> CGRTSCHLPRDVLTRACAYQDRRGQQRLPEWRDPDKYCPSYNKSPQSNSPVLLSRLHFEKDADSSERIIAPMRWGLVPSWFKESDPSKLQFNTTNCRSDTVMEKRSFKVPLGKGRRCVVLADGFYEWQRCQGTNQRQPYFIYFPQIKTEKSGSIGAADSPENWEKVWDNWRL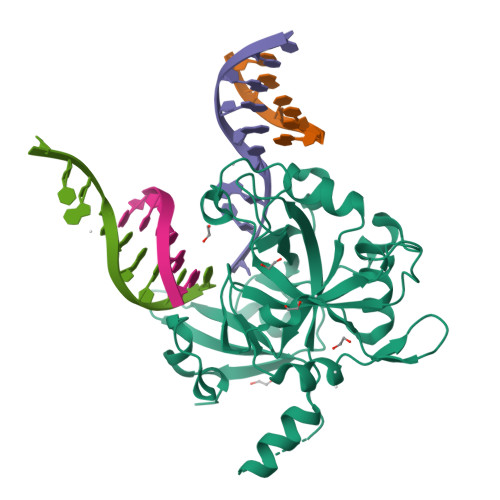LTMAGIFDCWEPPEGGDVLYSYTIITVDSCKGLSDIHHRMPAILDGEEAVSKWLDFGEVSTQEALKLIHPTENITFHAVSSVVNNSRNNTPECLAPVAENLYFQ> MHSSHHHHHHSSENLYFQGGGHMIHKLADVQSKNIGSGTRIWQFCVVLPSAIIGENCNICSH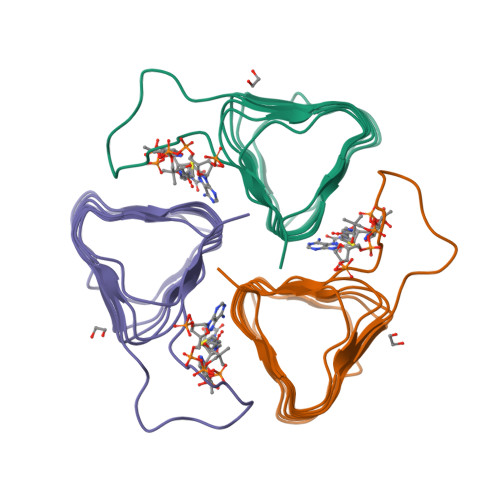CFIENDVKIGNNVTIKCGVQIWDGIEIEDDVFIGPNVTFCNDKYPRSKQYPKEFSKTIIKKGASIGANATILPGITIGENAMIGAGAIVTKDVLPHVTYYSKI> STSTIR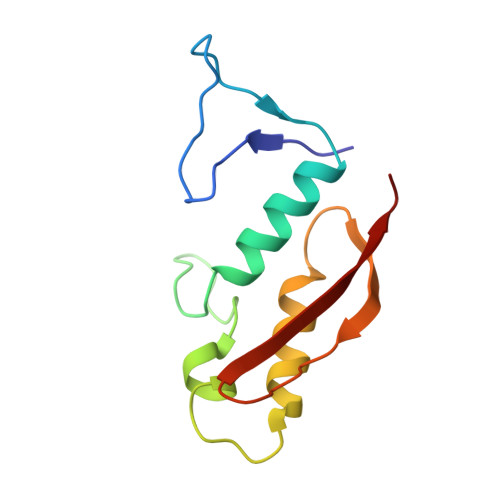TGTNNDILLDDNGNMVILRDVEACAQDVRAAMLMRTGENIFDVNSGVGYFEYIFSPQKSYDDARKSIADAILSSPDVTGIEQLDIDITGEVFGVDAKVITIH> MTETEIRLTGSPAPSFPQDRTCPYQPPKAYEERRGESPLTQVTLFDGRPAWLITGHAEGRALLVDPRLSSDWGHPDFPVVVRRTEDRGGLAFPLIGVDDPVHARQRRMLIPSFGVKRMNAIRPRLQSLVDRLLDDMLAKGPGADLVSAFALPVPSVAICELLGVPYGDHDFFEECSRNFVGAATSAEADAAFGELYTYLHGLVGRKQAEPEDGLLDELIARQLEEGDLDHDEVVMIALVLLVAGHETTVNAIALGALTLIQHPEQIDVLLRDPGAVSGVVEELLRFTSVSDHIVRMAKEDIEVGGATIKAGDAVLVSITLMNRDAKAYENPDIFDA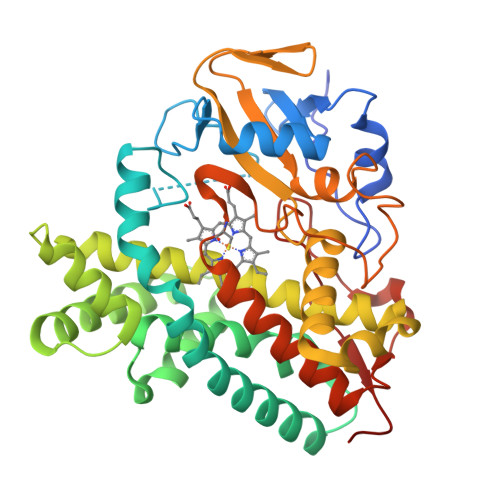RRNARHHVGFGHGIHQCLGQNLARAELEIALGGLFARIPGLRLAVPLDEVPIKAGHDAQGPIELPVVWHHHH> NPIA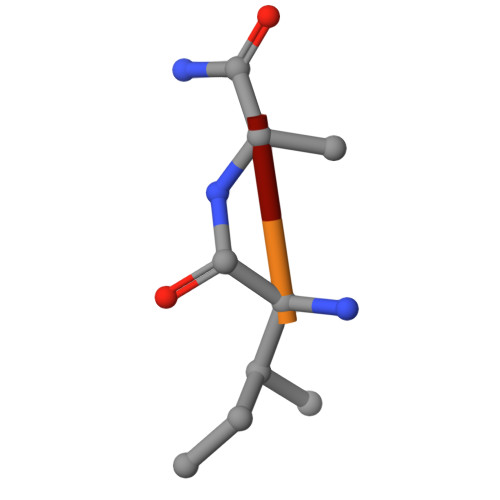A>[2x]MNHLGKTEVFLNRFALRPLNPEELRPWRLEVVLDPPPGREEVYPLLAQVARRAGGVTVRMGDGLASWSPPEVLVLEGTLARMGQTYAYRLYPKGRRPLDPKDPGERSVLSALARRLLQERLRRLEGVWVEGLAVYRREHARGPGWRVLGGAVLDLWVSDSGAFLLEVDPAYRILCEMSLEAWLAQGHPLPKRVRNAYDRRTWELLRLGEEDPKELPLPGGLSLLDYHASKGRLQGREGGRVAWVADPKDPRKPIPHLTGLLVPVLTLEDLHEEEGSLALSLPWEERRRRTREIASWIGRRLGLGTPEAVRAQAYRLSIPKLMGRRAVSKPAD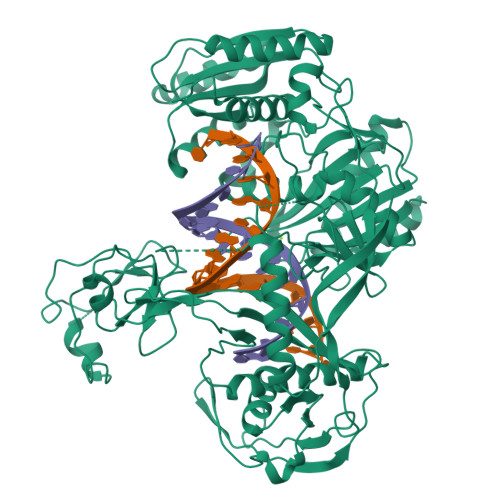ALRVGFYRAQETALALLRLDGAQGWPEFLRRALLRAFGASGASLRLHTLHAHPSQGLAFREALRKAKEEGVQAVLVLTPPMAWEDRNRLKALLLREGLPSQILNVPLREEERHRWENALLGLLAKAGLQVVALSGAYPAELAVGFNAGGRESFRFGGAACAVGGDGGHLLWTLPEAQAGERIPQEVVWDLLEETLWAFRRKAGRLPSRVLLLRDGRVPQDEFALALEALAREGIAYDLVSVRKSGGGRVYPVQGRLADGLYVPLEDKTFLLLTVHRDFRGTPRPLKLVHEAGDTPLEALAHQIFHLTRLYPASGFAFPRLPAPLHLADRLVKEVGRLGIRHLKEVDREKLFFV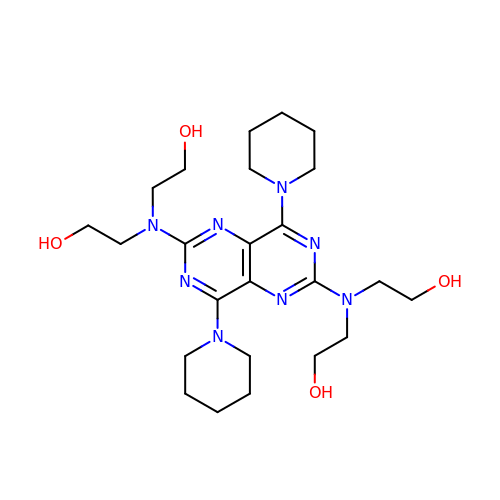2-[[2-[bis(2-hydroxyethyl)amino]-4,8-di(piperidin-1-yl)pyrimido[5,4-d]pyrimidin-6-yl]-(2-hydroxyethyl)amino]ethanol | C24 H40 N8 O4 | IZEKFCXSFNUWAM-UHFFFAOYSA-N> GAVKLNPDFSDAKENFYRVANWLVERWHFIMLNDTKRNTIYNAAIQKAVCLGSKSVLDIGAGTGILSMFAKKAGAHSVYACELSKTMYELACDVVAANKMEAGIK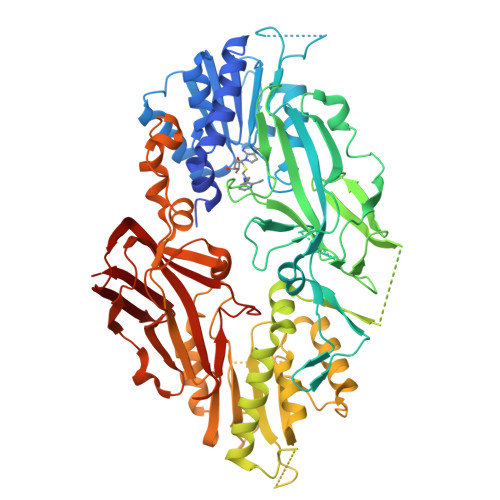LLHTKSLDIEIPKHIPERVSLVVTETVDAGLFGEGIVESLIHAWEHLLLQPKTKGESANCEKYGKVIPASAVIFGMAVECAEIRRHHRVGIKDIAGIHLPTNVKFQSPAYSSVDTEETIEPYTTEKMSRVPGGYLALTECFEIMTVDFNNLQELKSLATKKPDKIGIPVIKEGILDAIMVWFVLQLDDEHSLSTSPSEETCWEQAVYPVQDLADYWIKPGDHVMMEVSCQDCYLRIQSISVLGLECEMDVAKSFTQNKDLLSLGNEAELCSALANLQTSKPDAVEQTCILESTEIALLNNIPYHEGFKMAMSKVLSSLTPEKLYQTMDTHCQNEMSSGTGQSNTVQNILEPFYVLDVSEGFSVLPVIAGTLGQVKPYSSVEKDQHRIALDLISEANHFPKETLEFWLRHVEDESAMLQRPKSDKLWSIIILDVIEPSGLIQQEIMEKAAISRCLLQSGGKIFPQYVLMFGLLVESQTLLEENAVQGTERTLGLNIAPFINQFQVPIRVFLDLSSLPCIPLSKPVELLRLDLMTPYLNTSNREVKVYVCKSGRLTAIPFWYHMYLDEEIRLDTSSEASHWKQAAVVLDNPIQVEMGEELVLSIQHHKSNVSITVKQ> MPGGVSSPVRAFKSVGGQPIVFDHVKGAHIWDVDGNQYIDYVGSWGPAIVGHAHPEVIDALHAALEKGTSFGAPCLLENILAEMVIAAVPSVEMVRFVNSGTEACMAVLRLMRAYTQREKVIKFEGCYHGHADMFLVKAGSGVATLGLPDSPGVPKATTAATLTAPYNDLEAVSRLFEQYPNDIAGVILEPVV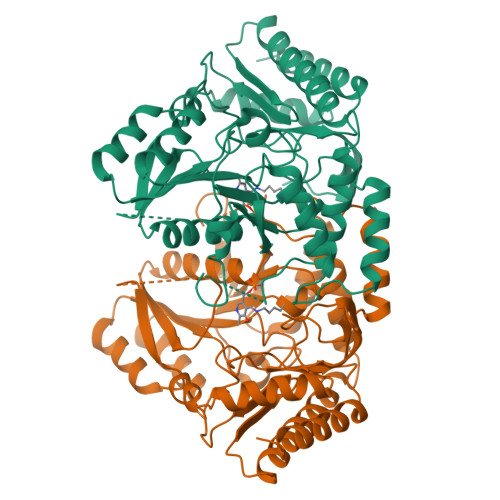GNAGFIPPDAGFLEGLRELTKQYGALLVFDEVMTGFRIAYGGAQEKFGVTPDLTTLGKVIGGGLPVGAYGGRAEIMKMVAPAGPVYQAGTLSGNPLAMTAGIKTLEILSRPGSYEHLDRITGKLVQGLLDAAREFGHEVCGGHISGMFGLFFTAGPVTNYEQAKQSDLKKFAAFHRGMLEQGIYLAPSQFEAGFTSLAHTEADIERTIAAARTVLSQL>GHMAEQELLAQPDAAYMDEAQQDFFRDLLLRQRQELQARIEGEFGELRDLERPSDEADLASREEQRQWQLRLLEREKKLLDKIDEALERLARGDYGWCQETGEPIGLRRLLLRPTATLCIEAKERQE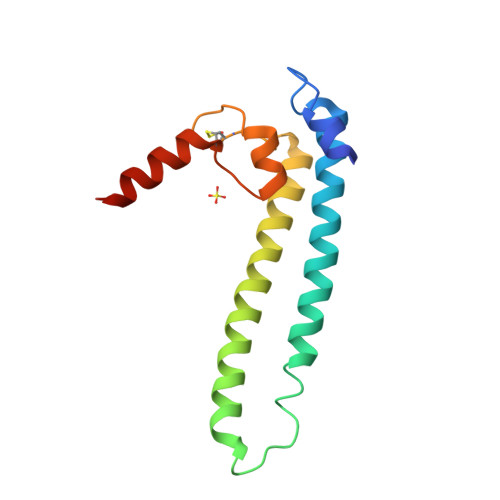KRERHVRHN[3x]> AWSHPQFEKVEAAPTAQQQLLEQVRLGEATHREDLVQQSLYRLELIDPNNPDVVAARFRSLLRQGDIDGAQKQLDRLSQLAPSSNAYKSSRTTMLLSTPDGRQALQQARLQATTGHAEEAVASYNKLFNGAPPEGDIAVEYWSTVAKIPARRGEAINQLKRINADAPGGSGSGSGVQGADAPVVAQNGPSRDVKLTFAQIAPPPGSMVLRGINPNGSIEFGMRSDEVVTKAMLNLEYTPSPSLLPVQSQLKVYLNDELMGVLPVTKEQLGKKTLAQMPINPLFISDFNRVRLEFVGHYQDVCEKPASTTLWLDVGRSSGLDLTYQTLNVKNDLSHFPVPFFDPSDNRTNTLPMVFAGAPDVGLQQASAIVASWFGSRSGWRGQNFPVLYNQLPDRNAIVFATNDKRPDFLRDHPAVKAPVIEMINHPQNPYVKLLVVFGRDDKDLLQAAKGIAQGNILFRGESVVVNEVKPLLPRKPYDAPNWVRTDRPVTFGELKTYEEQLQSSGLEPAAINVSLNLPPDLYLMRSTGIDMDINYRYTMPPVKDSSRMDISLNNQFLQSFNLSSKQEANRLLLRIPVLQGLLDGKTDVSIPALKLGATNQLRFDFEYMNPMPGGSVDNCITFQPVQNHVVIGDDSTIDFSKYYHFIPMPDLRAFANAGFPFSRMADLSQTITVMPKAPNEAQMETLLNTVGFIGAQTGFPAINLTVTDDGSTIQGKDADIMIIGGIPDKLKDDKQIDLLV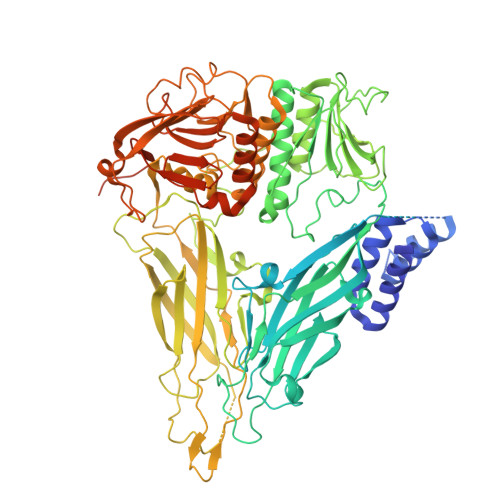QATESWVKTPMRQTPFPGIVPDESDRAAETRSTLTSSGAMAAVIGFQSPYNDQRSVIALLADSPRGYEMLNDAVNDSGKRATMFGSVAVIRESGINSLRVGDVYYVGHLPWFERVWYALANHPILLAVLAAISVILLAWVLWRLLRIISRRRLNPDNE> MHGAEH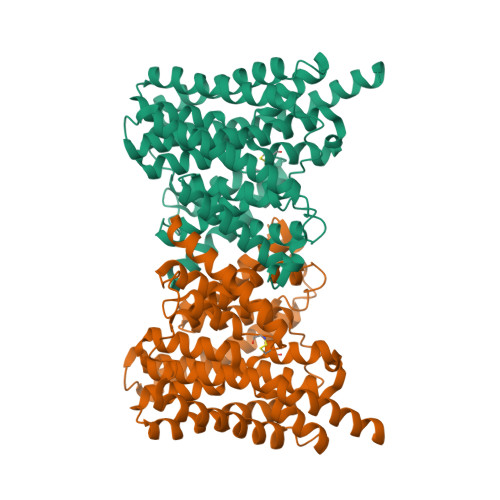LLEIFYLLLAAQVMAFIFKRLNQPCVIGEVLAGVLVGPALLGLVHEGEILEFLAELGAVFLLFMVGLETRLKDILAVGKEAFLVAVLGVALPFLGGYLYGLEIGFETLPALFLGTALVATSVGCTARVLQELGVLSRPYSRIILGAAVIDDVLGLIVLAVVNGVAETGQVEVGAITRLIVLSVVFVGLAVFLSTLIARLPLERLPVGSPLGFALALGVGMAALAASIGLAPIVGAFLGGMLLSEVREKYRLEEPIFAIESFLAPIFFAMVGVRLELSALASPVVLVAGTVVTVIAILGKVLGGFLGALTQGVRSALTVGVGMAPRGEVGLIVAALGLKAGAVNEEEYAIVLFMVVFTTLFAPFALKPLIAWTERERAAKE> DGDQSETSPSQNQGKCKDGLGEYTCTSL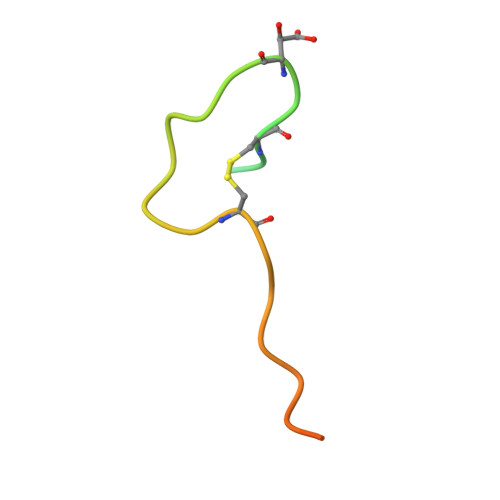EGFEGKNSELF>ASQPNSSAKKKEEKGKNIQVVVRCRPFNLAERKASAHSIVECDPVRKEVSVRTGGLADKSSRKTYTFDMVFGASTKQIDVYRSVVCPILDEVIMGYNCTIFAYGQTGTGKTFTMEGERSPNEEYTWEEDPLAGIIPRTLHQIFEKLTDNGTEFSVKVSLLEIYNEELFDLLNPSSDVSERLQMFDDPRNKRGVIIKGLEEITVHNKDEVYQILEKGAAKRTTAATLMNAYSSRSHSVFSVTIHMKETTIDGEELVKIGKLNLVDLAGSENIGRSGAVDKRAREAGNINQSLLTLGRVITALVERTPHVPYRESKLTRILQDSLGGRTRTSIIATISPASLNLEETLSTLEYAH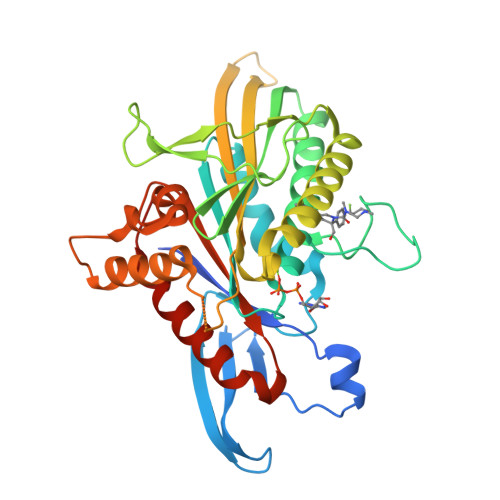RAKNILNKPEVNQK[2x]> SELLQRCESLEKKTATFENIVCVLNREVE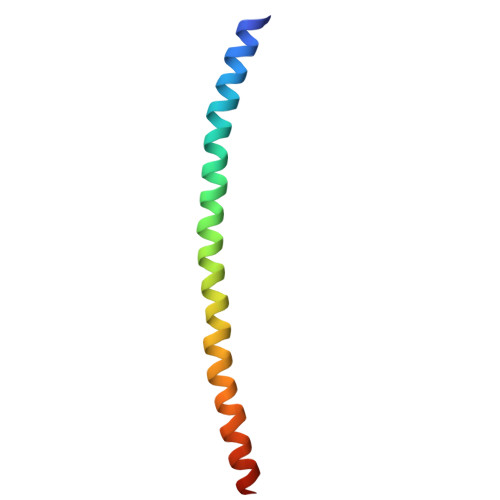RVAMTAEACSRQHRLDQDKIEALSSKVQQLERSIGLE>[4x]MDKELGKTLRRLRQGKQVSISSLADEHLSKSQISRFERGESEISCSRLLNLLDKLNITIDEFVSTHSKTHTHFFTLLSRVRKYYAEKNVAKLLKLLEDYAHKDYESTMIKAILSSIEPTVEPSEEEVTRLTDYLFSVEQWGYYEIILLGNCSRFINYNTLFLLTKEMVTSFAYSEQNKTNKTLVTQLSINCLIISIDYSYFDHSHYLIEKIEFLLRDE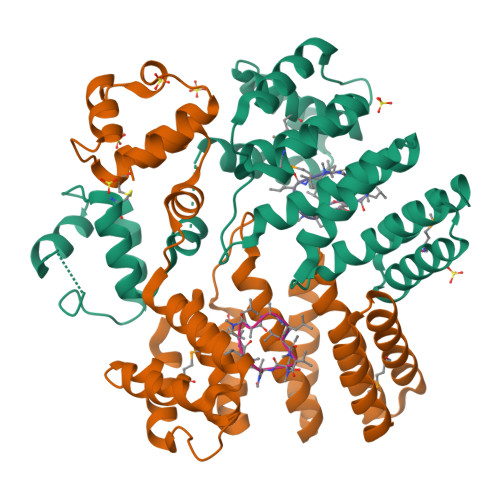LNFYEKTVFLYVHGYYKLKQGQVSGKDDMRQALQIFKYLGEDALYYSYKEHYRKEVLGDEEDEEEG;>ALLVTAGLVLA[4x]1-methyl-5-phenyl-6-{[(1R)-1-(pyridin-2-yl)ethyl]sulfanyl}-1,5-dihydro-4H-pyrazolo[3,4-d]pyrimidin-4-one | C19 H17 N5 O S | 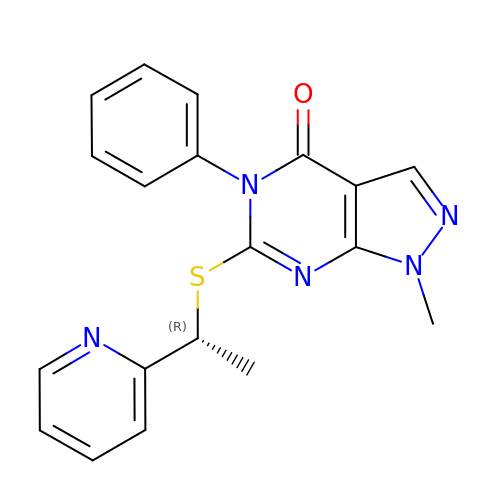DFGGDGDTSVXBMC-CYBMUJFWSA-N>[2x]GPSLGYCCGRKLEFSPQTLCCYGKQLCTIPRDATYYSYQNRYHFCEKCFNEIQGESVSLGDDPSQPQTTINKEQFSKRKNDTLDPELFVECTECGRKMHQICVLHHEIIWPAGFVCDGCLKKSARTRKENKFSAKRLPSTR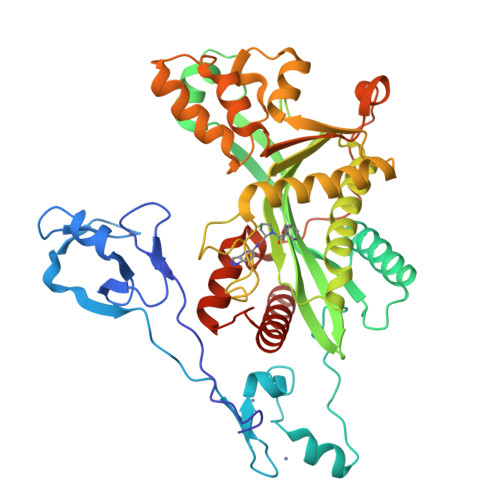LGTFLENRVNDFLRRQNHPESGEVTVRVVHASDKTVEVKPGMKARFVDSGEMAESFPYRTKALFAFEEIDGVDLCFFGMHVQEYGSDCPPPNQRRVYISYLDSVHFFRPKCLRTAVYHEILIGYLEYVKKLGYTTGHIWACPPSEGDDYIFHCHPPDQKIPKPKRLQEWFKKMLDKAVSERIVHDYKDIFKQATEDRLTSAKELPYFEGDFWPNVLEESIKESGGSGSQKLYATMEKHKEVFFVIRLIAGPAANSLPPIVDPDPLIPCDLMDGRDAFLTLARDKHLEFSSLRRAQWSTMCMLVELHTQSQDRF>MAEPLTVSPELTAN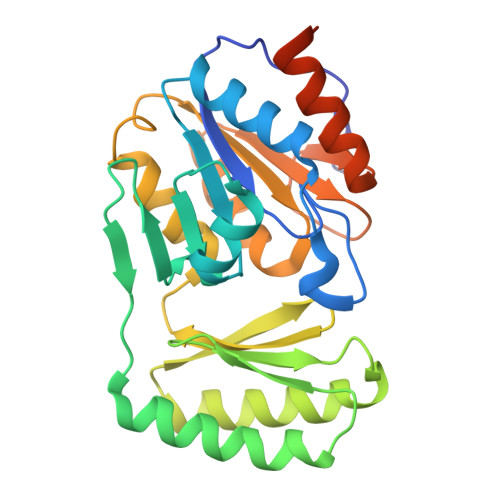YAYFFDLDGTLAEIKPHPDQVVVPHKILQLLDRLAAHNAGALALISGRSMTELDALAKPFRFPLAGVHGAERRDINGKTHIVRLPEAVVREVEALLRSTLVALPGTELESKGMAFALHYRQAPEHEAALLALAQHVTQHWPQLALQLGKCVVEIKPKGTNKGEAIAAFMQEAPFAGRIPVFVGDDLTDEAGFGVVNHAGGISVKVGVGATQAAWRLESVPDVWRWLEQINYPQQEQQVMNNRRDGYESFSRSI[2x]>[2x]GPGSMLDNIQEYLGVVKAKLTEFYEKVFQNFVKSLFGKPSSILFLGIDNAGKTTLVNKLKSDSTDVYMPTHHPSTSYIEIGNLKAQVIDLGGHTAARLAWRDYFYDCHGI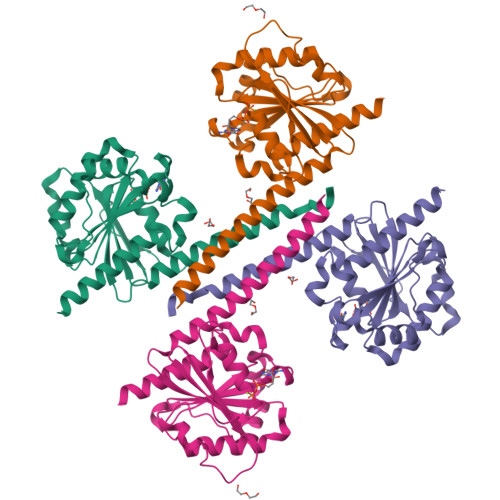VFIVDVHDVERFQEVREAYETVLSLEKRAPVVVLMNKIDLEGHTPETAEADYQWKSWLSQETGIENQEDPERGQVVKIFYVTITSGSANSITGPLARAFKWLEAMITYNNKKESL>[2x]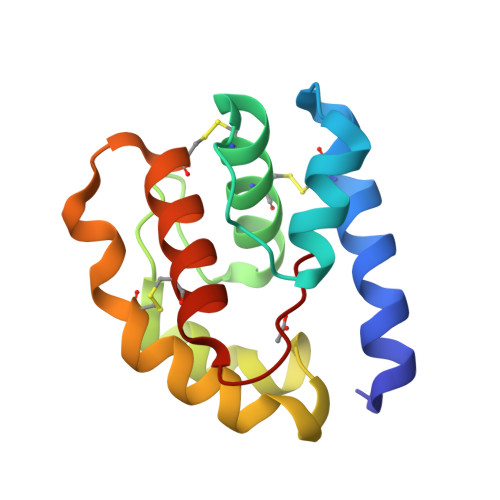MTMEQFLTSLDMIRSGCAPKFKLKTEDLDRLRVGDFNFPPSQDLMCYTKCVSLMAGTVNKKGEFNAPKALAQLPHLVPPEMMEMSRKSVEACRDTHKQFKESCERVYQTAKCFSENADGQFMWP>[2x]MAHHHHHHMSELKIKAAKAAIAYIEDDMVIGVGTGSTVN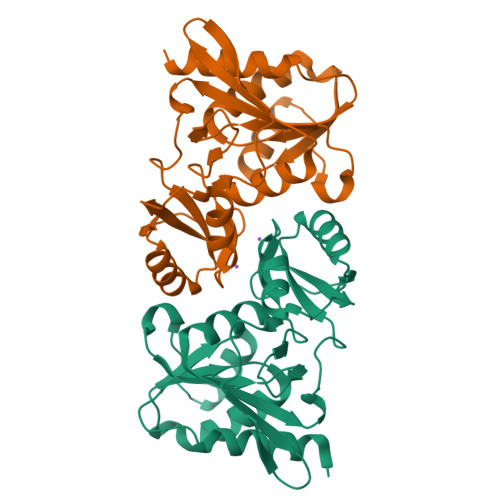FFIKELAAIKHKIEACVASSKATEALLRAEGIPVIDLNSVQDLPIYVDGADEVNERGEMIKGGGGALTREKIVANVATQFICIVDESKVVKRLGEFPVAVEVIPMARSFVARQIVKLGGDPEYREGFVTDNGNIILDVFNLSFSTPMALEDSLNVIPGVVENGVFAKRLADKVLVASASGVNNLK8-amino-N-[1-(cyclopropylcarbonyl)azetidin-3-yl]-2-(3-fluorophenyl)-1,7-naphthyridine-5-carboxamide | C22 H20 F N5 O2 | 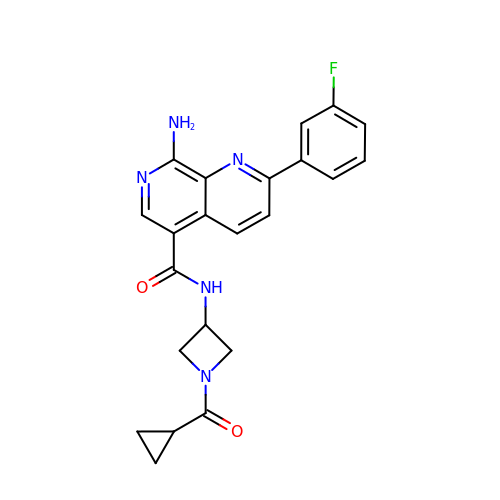FYXCIBJXJYBWPX-UHFFFAOYSA-N>NIKETLQKIKEVVLEIMDKGDDEQIKLAQSLLIVAEIAVAVGDKETVEKMYKEAKYILDNINSITDEEIKKMLEEAAKIAKKLLEKAKDLPEEERILLRIKALVIEVMAYGDDETIKEAQKLLIKAELAVKEGDLETLKKILKEMEKMVKEVK[4x];>[4x]DLEDLLEKIKDIVLKVMDIGDDETIKRAQKLLIKAELAVENKDLKEVEKLLKEAEKVYKEVKEA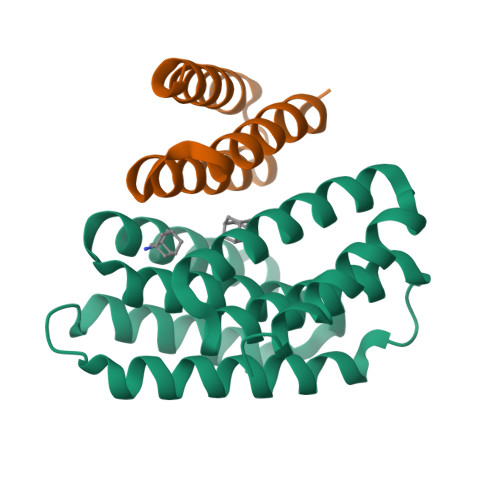K> GSEQLKHCNGILKELLSKKHAAYAWPFYKPVDASALGLHDYHDIIKHPMDLSTVKRKMENRDYRD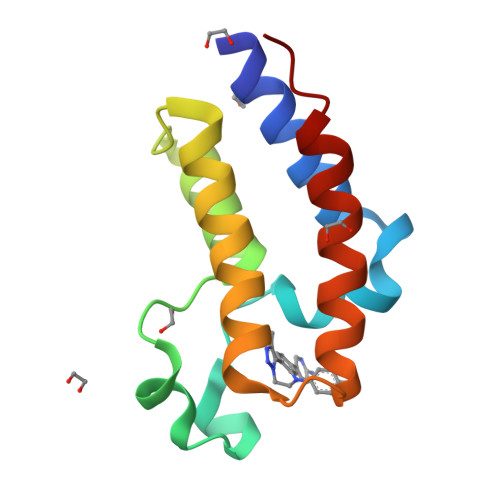AQEFAADVRLMFSNCYKYNPPDHDVVAMARKLQDVFEFRYAKMPD6-methyl-5-(4-phenyl-1,3-thiazol-2-yl)-2-(trifluoromethyl)pyridine-3-carboxylic acid | C17 H11 F3 N2 O2 S | 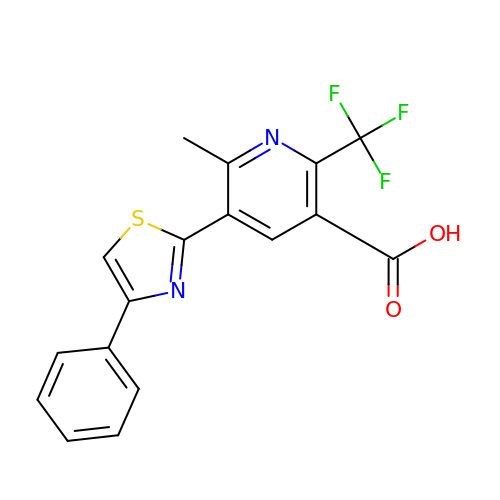AXBBYZUKIKQBNR-UHFFFAOYSA-N>GPDLVQKLKVLRHELSLQQPQAGHCRIEVSREEIFEESYRQIMKMRPKDLKKRLMVKFRGEEGLDYGGVAREWLYLLCHEMLNPYYGLFQYSTDNIYMLQINPDSSINPDHLSYFHFVGRIMGLAVFHGHYINGGFTVPFYKQLLGKPIQLSDLESVDPELHKSLVWILENDITPVLDHTFCVEHNAFGRILQHELKPNGRNVPVTEENKKEYVRLYVNWRFMRGIEAQFLALQKGFNELIPQHLLKPFDQKELELIIGGLDKIDLNDWKSNTRLKHCVADSNIVRWFWQAVETFDEERRARLLQF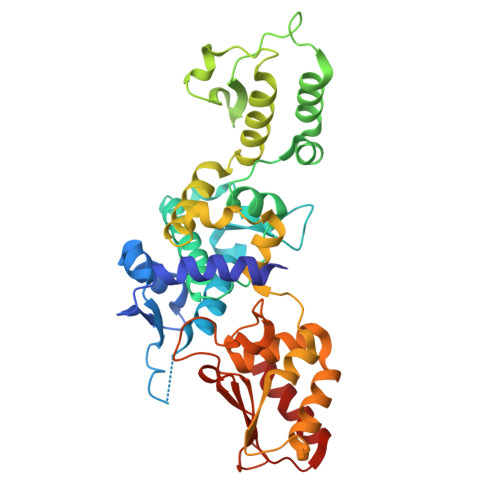VTGSTRVPLQGFKALQGSTGAAGPRLFTIHLIDANTDNLPKAHTCFNRIDIPPYESYEKLYEKLLTAVEET[4x]>[2x]PPYTIVYFPVRGRAEAMRMLLADQGQSWKEEVVTIDTWMQGLLKPTCLYGQLPKFEDGDLTLYQSNAILRHLGRSLGLYGKNQREAAQMDMVNDGVEDLRGKYV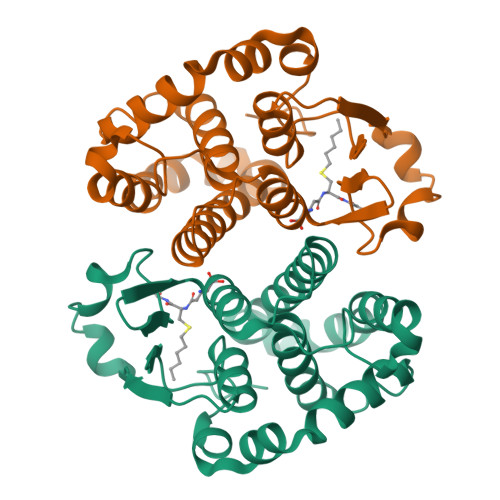TLIYTNYENGKNDYVKALPGHLKPFETLLSQNQGGKAFIVGDQISFADYNLLDLLLIHQVLAPGCLDNFPLLSAYVARLSARPKIKAFLSSPEHVNRPINGNGKQ>[8x]MSPSAPVNVTV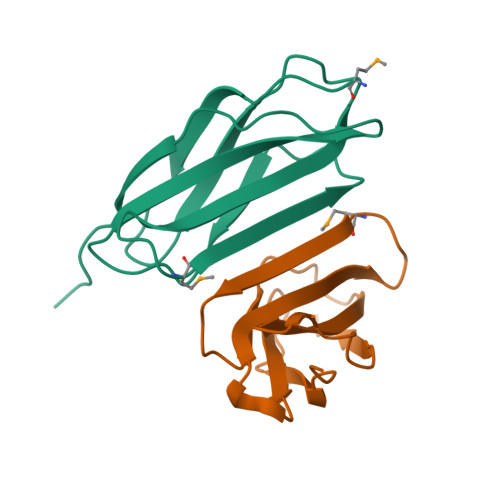RHLKANSAVVSWDVLEDEVVIGFAISQQKKDVRMLRFIQEVNTTTRSCALWDLEEDTEYIVHVQAISIQGQSPASEPVLFKTPREAEK> GAGCGACCTGTACGGACATCA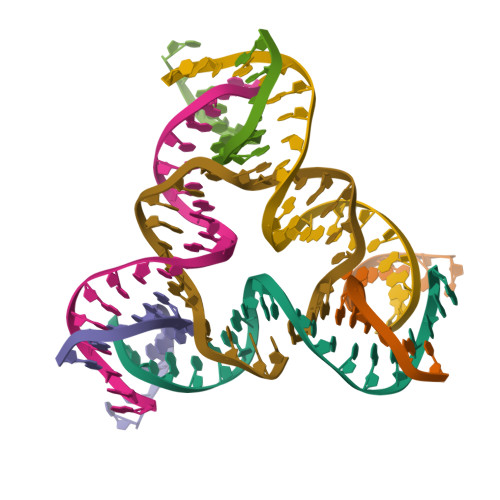;> AACCTACCTGGCAGGACGACT;> CACGAGCCTGATCGGACAAGA;> TCTGATGTGGTAGG;> TGTCTTGTGGTCGC;> TTAGTCGTGGCTCG;> ACACCGATCACCTGCCACCGT>[2x]FSNLAIYWGQGPNQLRLSHFCQETSLD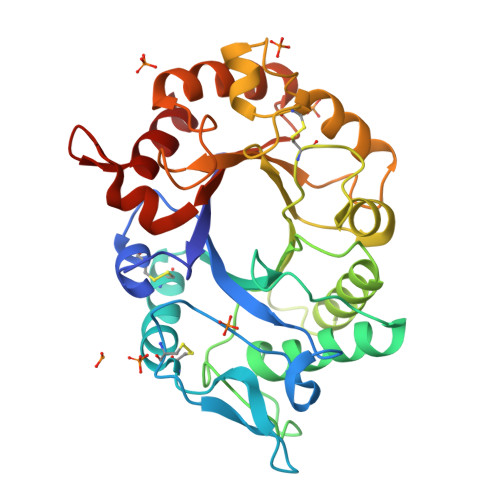IINIGFINYFPDMSPGHWPGSNFGNQCDGSVYVTNDGVVTKLLSGCHQIMEDIPICQAAGKKVLLSIGGAYPPDQSILSEDSAVAFATFLWGAFGPVAEGWEGPRPFGDVVVDGFDFDIEHNGGFGYATMVNTFRQYFNQVPERKFYLSAAPQCIIPDAQLSDAIFNAAFDFIWIQYYNTAACSAKSFIDTSLGTFNFDAWVTVLKASASKDAKLYVGLPASETAANQGYYLTPDEVESLVSTYMDRYPDTFGGIMLWEATASENNQIDGAPYADHMKDILLH4-[4-(quinolin-2-yl)-1H-1,2,3-triazol-1-yl]phenol | C17 H12 N4 O | 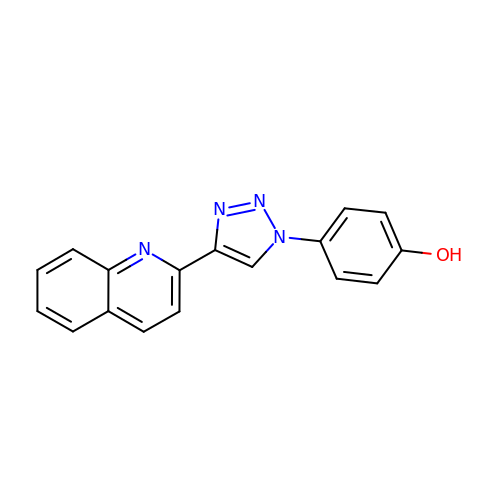QSDNOMVFORBNKO-UHFFFAOYSA-N> MDETVAEFIKRTILKIPMNELTTILKAWDFLSENQLQTVNFRQRKESVVQHLIHLCEEKRAS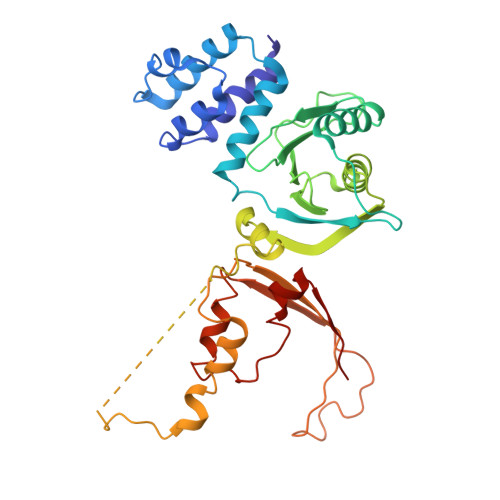ISDAALLDIIYMQFHQHQKVWEVFQMSKGPGEDVDLFDMKQFKNSFKKILQRALKNVTVSFRETEENAVWIRIAWGTQYTKPNQYKPTYVVYYSQTPYAFTSSSMLRRNTPLLGQALTIASKHHQIVKMDLRSRYLDSLKAIVFKQYNQTFETHNSTTPLQERSLGLDINMDSRIIHENIVEKERVQRITQETFGDYPQPQLEFAQYKLETKFKSGLNGSILAEREEPLRCLIKFSSPHLLEALKSLAPAGIADAPLSPLLTCIPNKRMNYFKIRDK> D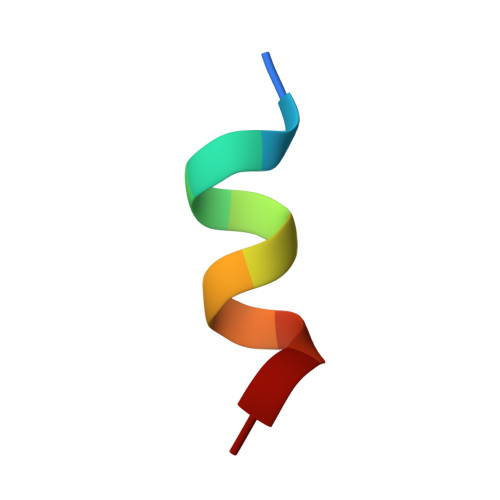HQLLRYLLDK>PMFIVNTNVPRASVPDGFLSELTQQLAQATGKPPQYIAVHVVPDQLMAFGGSSEPCALCSLHSIGKIGGAQNRSYSKLLCGLLAERLRISPDRVYINYYDMNAANVGWNNS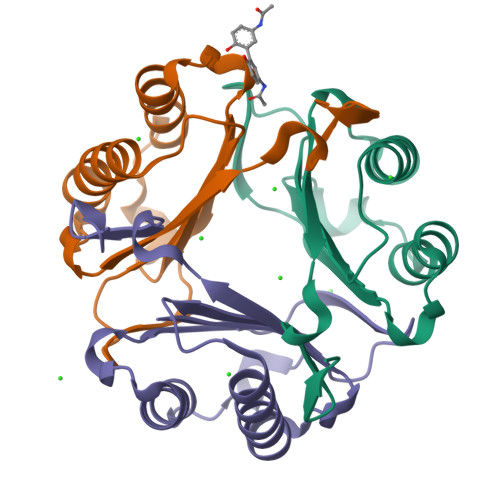TFA[6x]> ANVRLQHHHHHHHLEAEAFSSESKWMTGDWGGTRTELLDKGYDFTLDYVGEVAGNLHGGYNDDKTARYSDQFALGAHLDLQKILGWHDAEFKLAITERSGRNLSNDRISDPRAGQFSSVQEVWGRGQTWRLTQMWIKQKYFDGALDVKFGRFGEGEDFNSFPCDFQNLAFCGSQVGNWVGGIWYNWPVSQWALRVKYNITPAFFVQVGAFEQNPSNLETGNGFKLSGSGTKGAIMPMEAVWSPKVNGLPGEYRLGYYYSTAKADDVYDDVNGNPQALTGEAFKSHSSKHGWWVVAQQQVTAHGGDVNRGLSLFANFTVHDKATNVVDNYQQVGLVYKGAFDARPKDDIGFGVARIHVNDDVKKRAELLNAQSGINDYDNPGFVPLQRTEYNAELYYGFHVTNWLTVRPNLQYIKSPGGV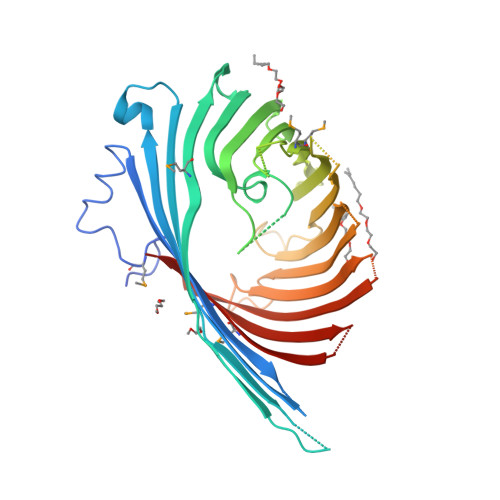DEVDNALVAGMKMQSSF>MDVLRTPDERFTALPDFPFAPRYV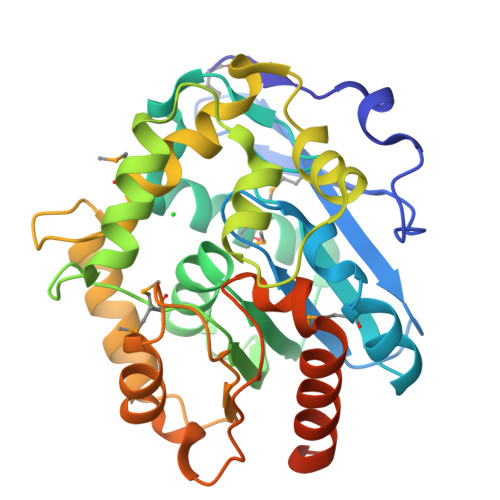EVDSGDGGTLRMHYLDEGRSDGEVVLLLHGEPSWSYLYRWMIPVLVEAGLRAVAIDLVGFGRSDKPTSRDDYTYQAHVDWMWAAIEEIGLADVTLVCQDWGGLIGLRLVGEHPDRFARVVAANTMLPTGDHHPGEAFLAWQKFSQEVPLFPAGQIVNGGSLSTLSAETIAAYDAPFPDASYQAGARQFPMLVPISPDDPATPANRKAWAALGRFEKPFLSAFSDSDPITGAAEPVLRGHVPGARGQSHVTIAGAGHFLQEDKGRELAEAVVTFVRANPRAELNSSSVDKLAAALEHHHHHH[4x]> MERTELLKPRTLADLIRILHELFAGDEVNVEEVQAVLEAYESNPAEWALYAKFDQYRYTRNLVDQGNGKFNLMILCWGEGHGSSIHDHTDSHCFLKLLQGNLKETLFDWPDKKSNEMIKKSERTLRENQCAYINDSIGLHRVENVSHTEPAVSLHLYSPPFDTSHAFDQRTGHKNKVTMTFHSKFGIRTPFTTSGSLE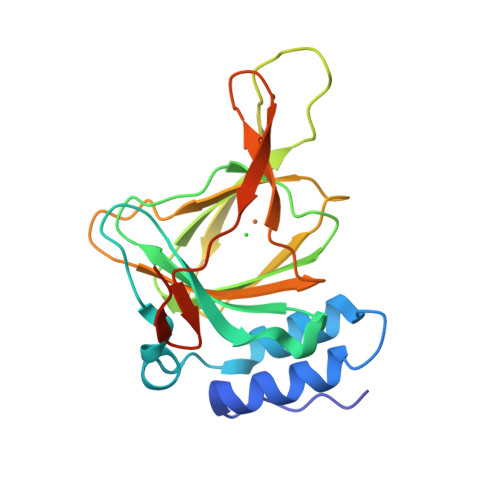NN>[2x]EDADKLPHTKVTLVAPPQVHPHEQATKSGPKVVEFTMTIEEKKMVIDDKG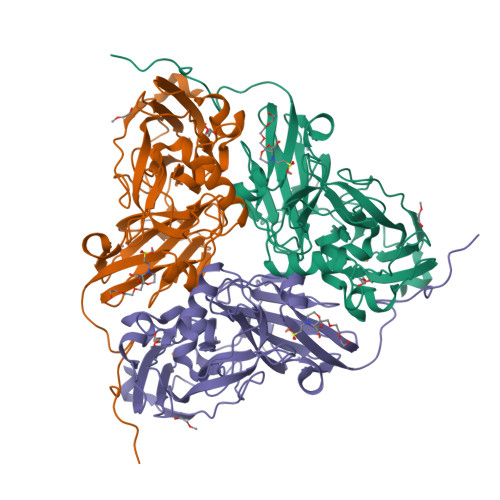TTLQAMTFNGSMPGPTLVVHEGDYVQLTLVNPATNAMPHNVDFHGATGALGGAKLTNVNPGEQATLRFKADRSGTFVYHCAPEGMVPWHVVSGMSGTLMVLPRDGLKDPQGKPLHYDRAYTIGEFDLYIPKGPDGKYKDYATLAESYGDTVQVMRTLTPSHIVFNGKVGALTGANALTAKVGETVLLIHSQANRDTRPHLIGGFGDWVWETGKFANPPQRDLETWFIRGGSAGAALYTFKQPGVYAYLNHNLIEAFELGAAGHIKVEGKWNDDLMKQIKAPAPIPR> MDSTNLNKRPLLQYSLSSLGSQITKWSSSRPTSPVRKARSTENDFLSKQDTSSILPSINDDGGEQWYEKFKPNCLEQVAIHKRKLKDVQEALDAMFLPNAKHRILLLSGPSGCSKSTVIKELSKILVPKYRQNSNGTSFRSTPNEHKVTEFRGDCIVNDLPQMESFSEFLKGARYLVMSNLSLILIEDLPNVFHIDTRRRFQQLILQWLYSSEPLLPPLVICITECEIPENDNNYRKFGIDYTFSAETIMNKEILMHPRLKRIKFNPINSTLLKKHLKFICVQNMKMLKEKNKWNKRQEVIDYIAQETGDIRSAITTLQFWATSSGSLPISTRESTISYFHAIGKVIHGSHSTNNDNEMINNLFENSNNLLSKEDFKLGILENYNTFNKGEFSISDASSIVDCLSECDNMNGLPESNEYGLREVRKTFRNISKQGHNHGTVYFPREWKVRKLQNSFKVQAEDWLNVSLYKYNAVHSFRNITLEFGYYAPLIRKCQSYKKKYILYYLKNLPSGSSGPKQTMDKFSDIMKVENGIDVVDRIGGPIEALSVEDGLAPLMDNDSNNCDHLEDQKKERDRRLRMLIDQYERNVMMANDDLEDEETSFNDDPIVDSDSDNSNNIGNETFGRSDEDESLCEILSQRQPRKAPVISESLSDSDLEIL;> MSKTLSLQLPWVEKYRPQVLSDIVGNKETIDRLQQIAKDGNMPHMIISGMPGIGKTTSVHCLAHELLGRSYADGVLELNASDDRGIDVVRNQIKHFAQKKLHLPPGKHKIVILDEADSMTAGAQQALRRTMELYSNSTRFAFACNQSNKIIEPLQSRCAILRYSKLSDEDVLKRLLQIIKLEDVKYTNDGLEAIIFTAEGDMRQAINNLQSTVAGHGLVNADNVFKIVDSPHPLIVKKMLLASNLEDSIQILRTDLWKKGYSSIDIVTTSFRVTKNLAQVKESVRLEMIKEIGLTHMRILEGVGTYLQLASMLAKIHKLNNKA;> MSTSTEKRSKENLPWVEKYRPETLDEVYGQNEVITTVRKFVDEGKLPHLLFYGPPGTGKTSTIVALAREIYGKNYSNMVLELNASDDRGIDVVRNQIKDFASTRQIFSKGFKLIILDEADAMTNAAQNALRRVIERYTKNTRFCVLANYAHKLTPALLSRCTRFRFQPLPQEAIERRIANVLVHEKLKLSPNAEKALIELSNGDMRRVLNVLQSCKATLDNPDEDEISDDVIYECCGAPRPSDLKAVLKSILEDDWGTAHYTLNKVRSAKGLALIDLIEGIVKILEDYELQNEETRVHLLTKLADIEYSISKGGNDQIQGSAVIGAIKASFENETVKANV;> MFEGFGPNKKRKISKLAAEQSLAQQPWVEKYRPKNLDEVTAQDHAVTVLKKTLKSANLPHMLFYGPPGTGKTSTILALTKELYGPDLMKSRILELNASDERGISIVREKVKNFARLTVSKPSKHDLENYPCPPYKIIILDEADSMTADAQSALRRTMETYSGVTRFCLICNYVTRIIDPLASRCSKFRFKALDASNAIDRLRFISEQENVKCDDGVLERILDISAGDLRRGITLLQSASK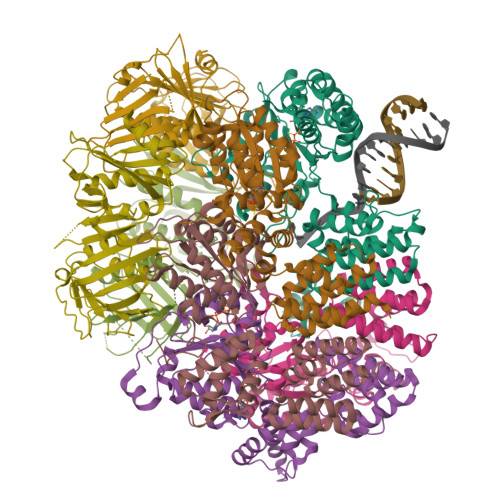GAQYLGDGKNITSTQVEELAGVVPHDILIEIVEKVKSGDFDEIKKYVNTFMKSGWSAASVVNQLHEYYITNDNFDTNFKNQISWLLFTTDSRLNNGTNEHIQLLNLLVKISQL;> MSLWVDKYRPKSLNALSHNEELTNFLKSLSDQPRDLPHLLLYGPNGTGKKTRCMALLESIFGPGVYRLKIDVRQFVTASNRKLELNVVSSPYHLEITPSDMGNNDRIVIQELLKEVAQMEQVDFQDSKDGLAHRYKCVIINEANSLTKDAQAALRRTMEKYSKNIRLIMVCDSMSPIIAPIKSRCLLIRCPAPSDSEISTILSDVVTNERIQLETKDILKRIAQASNGNLRVSLLMLESMALNNELALKSSSPIIKPDWIIVIHKLTRKIVKERSVNSLIECRAVLYDLLAHCIPANIILKELTFSLLDVETLNTTNKSSIIEYSSVFDERLSLGNKAIFHLEGFIAKVMCCLD;> MKLKLIVNGCEAPDDYKLLRTTINTVASLRKTAILRFNSERLTIISTPKSSLNSSNNGTILRGDTGQLWCTIPHDVFRLYTVISARELNTITMECNCDSLLSVFKRYDRVMNQGSSSNMTIKLQSMPEWNTNNGTLSGGTAGGVDTTSKPNPICALGITFEEIVHTSGPNDAIVMNGGVDEHNGLPTTVGTGNLLASNKVIMHSFKVPVKLLFRAQDTRIQEPMINYIQLMMYKLPPISGEFGSAFHGFIRRVERYSNVNHIHLMGVKKKEHGNEGDDVELKIIVNELDWHLEICWNGPLDSVIQRQEGLTDNPSQNQHIDTDGRQEEGSLPIIEADKPMSSLYTNTRDREMEENIRYDEDLLRIEDSSIADTRGNIYTADTSGDTEFNDISVMVEKAEQESSSTHEVIIRCKDWKVCSKLYAAFEEVVLAISHDESCVFHCSLDERGQIIYYIARSKGL;> MRINSELANKFSASTVHLEHITTALSCLTPFGSKDDVLIFIDADGLSFVRENNHVIKIQLLLSRELFMSYSYRNETEDHMKLCVKINHILDSVSVMNRNSDDIVECTLSYDGHGSPFVLIFEDSFISERVEYSTYLIKDFDTNGLELDRERISFEAIIKGEALHSALKDLKEIGCKECYVYAKTEANDENVFALISKSQLGFSKIKLPSNRSILEKLQVFDGDSTTVIDGFAVIGFFDFTSFDKIRKSTKIASKVLFRMDVHGVLSVNILSQTDDVIITDTTRPSNNRPGSIRQLQLPKDYPGIVIEVCMLEKESIDEAAQTEIELLMETNELGNRNSFKKSTIRKRYGTDKGNETSNDNLLQLNGKKIKLPSEEENNKNRESEDEENHCKYPTKDIPIFF;> MSFKATITESGKQNIWFRAIYVLSTIQDDIKITVTTNELIAWSMNETDTTLCQVRFQKSFFEEYEFKPHEIVFGENGVQVIEDTYGNSHKLYSFRVNGRHLTTISRKPDGDGIKSFTIAVNNTSTCPESLANRLIVVIEMDSLIVKEYCPQFQPIKYDPIIINLKYKRRFLDVFGTAASDRNPQEPLDPKLLDVFTNTERELTSALFNEEVESDIRKRNQLTAADEINYICCNSTLLKNFLDNCNVNVTDEVKLEINVHRLSITAFTKAVYGKNNDLLRNALSMSNTISTLDLEHYCLFTKSIIFKLKDFKNFITIGPSWKTTQDGNDNISLWFCHPGDPILMQMQKPGVKLELVEVTDSNINDDILEGKFIKTAISGSKEEAGLKDNKESCESPLKSKTALKRENLPHSVAGTRNSPLKVSYLTPDNGSTVAKTYRNNTARKLFVEEQSQSTNYEQDKRFRQASSVHMNMNREQSFDIGTTHEVACPRNESNSLKRSIADICNETEDPTQQSTFAKRADTTVTWGKALPAADDEVSCSNIDRKGMLKKEKLKHMQGLLNSQNDTSNHKKQDNKEMEDGLGLTQVEKPRGIFD> MNRNPDQNTLPNITLKIIETYLGRVPSVNEYHMLKSQARNIQKITVFNKDIFVSLVKKNKKRFFSDVNTSASEIKDRILSYFSKQTQTYNIGKLFTIIELQSVLVTTYTDILGVLTIKAPNVISSKISYNVTSMEELARDMLNSMNVAVIDKAKVMGRHNVSSLVKNVNKLMEEYLRRHNKSCICYGSYSLYLINPNIRYGDIDILQTNSRTFLIDLAFLIKFITGNNIILSKIPYLRNYMVIKDENDNHIIDSFNIRQDTMNVVPKIFIDNIYIVDPTFQLLNMIKMFSQIDRLEDLSKDPEKFNARMATMLEYVRYTHGIVFDGKRNNMPMKCIIDENNRIVTVTTKDYFSFKKCLVYLDENVLSSDILDLNADTSCDFESVTNSVYLIHDNIMYTYFSNTILLSDKGKVHEISARGLCAHILLYQMLTSGEYKQCLSDLLNSMMN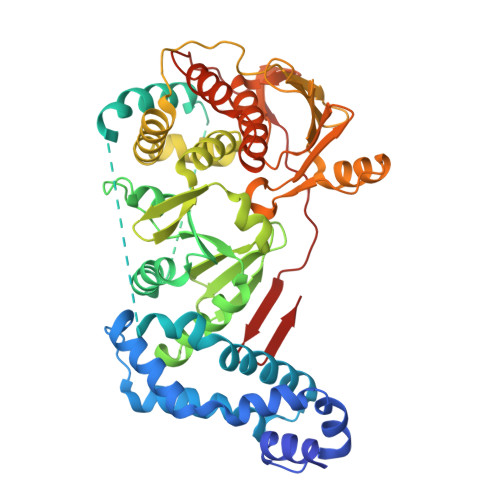RDKIPIYSHTERDKKPGRHGFINIEKDIIVF>[2x]GPLGSNKVHRAPELVEFYQSLMKRESKKEGAPSLISSGTGNSSAARNNMIGEIENRSTFLLAVKADVETQGDFVQSLATEVRASSFTDIEDLLAFVSWLDEELSFLVDERAVLKHFDWPEGKADALREAAFEYQDLMKLEKQVTSFVDDPNLSCEPALKKMYKLLEKVEQSVYALLRTRDMAISRYKEFGIPVDWLSDT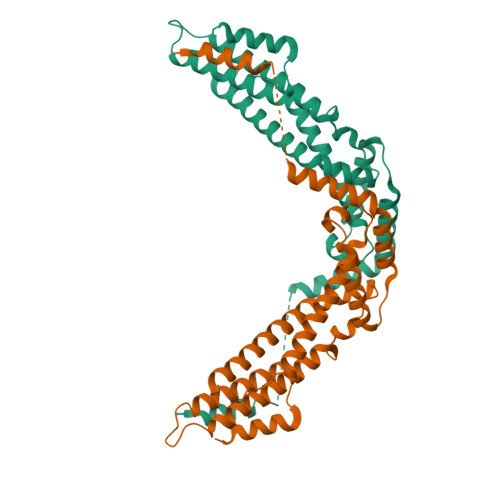GVVGKIKLSSVQLAKKYMKRVAYELDSVSGSDKDPNREFLLLQGVRFAFRVHQFAGGFDAESMKAFEELRSRA>[2x]AEEELPPRKVCIVGAGVSGLYIAMILDDLKIPNLTYDIFESSSRTGGRLYTHHFTDAKHDYYDIGAMRYPDIPSMKRTFNLFKRTGMPLIKYYLDGENTPQLYNNHFFAKGVVDPYMVSVANGGTVPDDVVDSVGE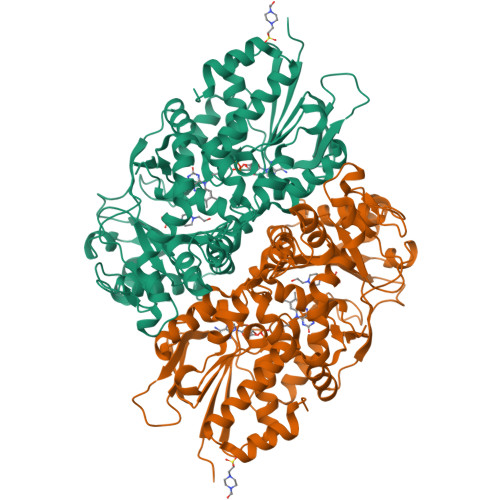KLQQAFGYYKEKLAEDFDKGFDELMLVDDMTTREYLKRGGPKGEAPKYDFFAIQWMETQNTGTNLFDQAFSESVIDSFDFDNPTKPEWYCIEGGTSLLVDAMKETLVHKVQNNKRVEAISIDLDAPDDGNMSVKIGGKDYSGYSTVFNTTALGCLDRMDLRGLNLHPTQADAIRCLHYDNSTKVALKFSYPWWIKDCGITCGGAASTDLPLRTCVYPSYNLGDTGEAVLLASYTWSQDATRIGSLVKDAPPQPPKEDELVELILQNLARLHAEHMTYEKIKEAYTGVYHAYCWANDPNVGGAFALFGPGQFSNLYPYLMRPAAGGKFHIVGEASSVHHAWIIGSLESAYTAVYQFLYKYKMWDYLRLLLERWQYGLQELETGKHGTAHLQFILGSLPKEYQVKIV> MNK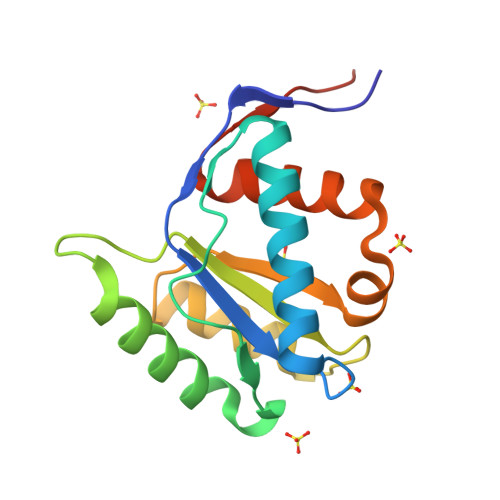KMINGGTVNNWICINFSRQVQDNLARTFCQELAQMCYVSGMAFNPEPVLPPVSARPEQVEKVLKTRYHDATSKLSQGKEIDLLIVILPDNNGSLYGDLKRICETELGIVSQCCLTKHVFKMSKQYMANVALKINVKVGGRNTVLVHHHHHH> MASMTGGQQMGAPITAYAQQTRGLLGCIITSLTGRDKNQVEGEVQIVSTATQTFLATCINGVCWTVYHGAGTRTIASPKGPVIQMYTNVDQDLVGWPAPQGSRSLTPCTCGSSDLYLVTRHADVIPVRRR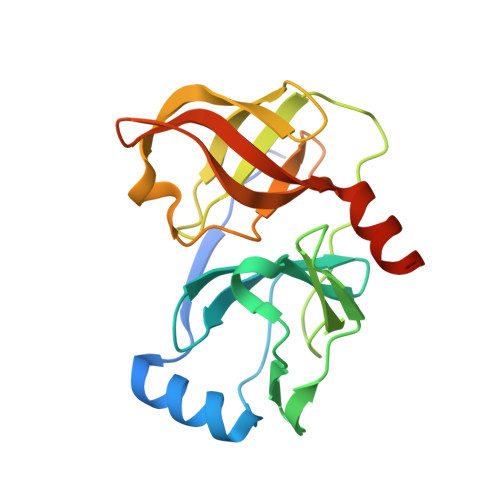GDSRGSLLSPRPISYLKGSSGGPLLCPAGHAVGLFRAAVCTRGVAKAVDFIPVENLETTMRSGSHHHHHH> XXXXXXXXXXXXXMSSEDIIYDPQFKPVQGIYENRLRQFIDTGGDYHDLNLPKFYDKKRISLDHDHVKVWWYQVSFERGSSPVSPDKRPSWKSIIERDKKGELEFREANINQPFGPSWSTTWFKVKISLPEDWVKSNEQLLFQWDCSNEGIVIDPKTLIPVTAFSGGERTEYVLPKTSDGKHFFYIEAGNNGMFGCGAGSTINPPDDNRFFHLRKADIVWPDLDARALYIDFWMLGDAARELPGDSWQKHQARQLGNAVMNLFDPNDRSSVRKCRELLQREYFDSFLESSKVYEQGESQVLTNVYGIGNCHIDTAWLWPFAETRRKIVRSWSSQCTLMDRFPEYKFVASQAQQFKWLLEDHPEFFNKVLIPKIQQSQFFAVGGTWVENDTNIPSGESLARQFFFGQRFFLKHFGLKSKIFWLPDTFGYSSQMPQLCRLSGIDKFLTQKLSWNNINSFPHSTFNWAGIDGSQLLTHMPPGNTYTADSHFGDVLRTAKQNKTPEYYGSGLMLYGKGDGGGGPTEEMLQKMRRIRSMNNRNGNVIPKLQVGITVDEFYDDILKRTNQGHDLPTWSGELYFEFHRGTYTSQAQTKKLMRLSEIKLHDLEWIAAKTSVLYPDSYKYPSKQINELWENVLLCQFHDVLPGSCIEMVYKYEAVPMLHNVVKECTSLIDKTVQFLQSQSKADLVEMRTLTWSKPEKVSEECSLNGSYTSSVTGYDDYIVLANGKLKVIICKKTGVITSITDETLGVEYLDTEHGRNKLGANQFVIYDDKPLGWQAWDTELYSVNQYKYVTKPKKVQVSCNTKEKCAVEVIFQISEKCKIKSVISLNATAVTDAKLSKVDISTTVENWDARNKFLKVEFPVNIRNDFASYETQFGITKRPTHYNTSWDVAKFEVCHHKFADYSEYSKGVSILNDCKYGFSTHGNLMRLSLLRSPKAPDAHADMGTHEIKYAIYPHRGALSSDTVKLAHEFNYCFKYKLPKDIGMNFDDIISISGDENVILSNIKRGEDDSAVKSNYSLNPRDEQSIVVRVYESLGGESFASLNTTLNLKRIEKVDNLEMKVYKSLTATRDESNHAINRIPIKLRPFEIASFRLYF

The earliest discovered selective autophagy pathway in Saccharomyces (S.) cerevisiae is the cytoplasm‐to‐vacuole targeting (Cvt) pathway, through which hydrolytic enzymes are sequestered into double‐membrane vesicles, termed Cvt vesicles, and transported to the vacuole 8, 9. The best‐characterized cargo component of the Cvt vesicle is the vacuolar aminopeptidase I (Ape1) 16. Ape1 is synthesized in the cytosol as a 55‐kDa zymogen that includes an N‐terminal propeptide (hereafter referred to as prApe1), which oligomerizes into a dodecamer 17, 18 and further assembles into larger aggregates in a propeptide‐dependent manner 19. In addition to prApe1, Atg19 also binds another cargo hydrolase α‐mannosidase 1 (Ams1) 25, 26 via a site distinct from the prApe1 binding site, thus forming the Cvt complex.

In order to further the structural analysis of the components in Cvt vesicles, we determined the 3D structure of the secondary cargo Ams1 from S. cerevisiae using cryo‐EM. The images revealed class average views with two perpendicular twofold rotation axes indicative of dihedral symmetry and were used for determination of an initial low‐resolution 3D model of Ams1. After vitrification of the sample, we refined the tetrameric Ams1 structure to 6.3 Å overall resolution from 33,588 particles (and EV3A). Subsequently, we built a complete pseudo‐atomic model based on a homology model of the mannosidase core combined with two additional N‐terminal domains. For the remaining N‐terminus, we built two domains: a jelly‐roll fold (residues 45–203) and a four‐helix bundle (residues 17–27, 209–271) based on distant homology and the EM density (Movie EV1). In contrast to the homologous dimeric S. pyogenes α‐mannosidase 32, S. cerevisiae Ams1 forms a tetramer. The transverse interface connecting two monomers perpendicularly to the Ams1 length axis is formed by the β‐sandwich domain and is located on the opposite side of the dimerization interface described in the homologous mannosidase structure (and Movie EV1). In addition, we identified an N‐terminal four‐helix bundle domain that comprises the major longitudinal interface bridging two monomers along the Ams1 length axis within the tetramer. In analogy to the mApe1 structure, a putative Zn2+ ion is coordinated by central enzymatic residues of Ams1 His298, Asp300, Asp411, His626, and is located in the interior of the oligomeric assembly. The corresponding SDS–PAGE shows that wild‐type tetrameric Ams1 binds MBP‐Atg19 efficiently, whereas the introduction of a W234E mutation drastically reduces binding (Fig EV3E). This suggests that the Ams1 wild‐type tetramer is required for in vitro recognition by the autophagy receptor Atg19.>[4x]MAFELPNLPYGFRALEPHIDQQTMEIHHDKHHNTYVTRLNAAVEGTDLESKSIEEIVANLDSVPENIQTAVRNNGGGHLNHSLFWELLTPNSEEKGTVVDKIKEQWG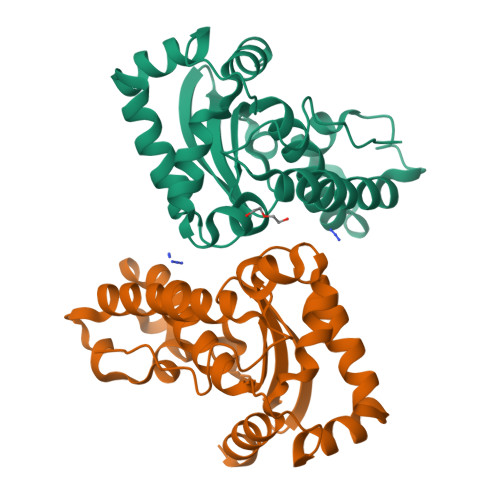SLDAFKEEFANQAEARFGSGWAWLVVNDGKLEIVTTPNQDNPLTEGKTPILGLDVWEHAYYLKYQNKRPDYISAFWNVVNWEKVDELYNAAKHHHHHH>AAMAGGEGNMSASATETNARVFSLHLGATRVVYNPASSGETLTVINDQDYPMLVQSEVLSEDQKSPAPFVVTPPLFRLDGQQSSRLRIVRTGGEFPPDRESLQWICVKGIPPKEGDRWAEGKDGEKKADKVSLNVQLSVSSCIKLFVRPPAVKGRPDD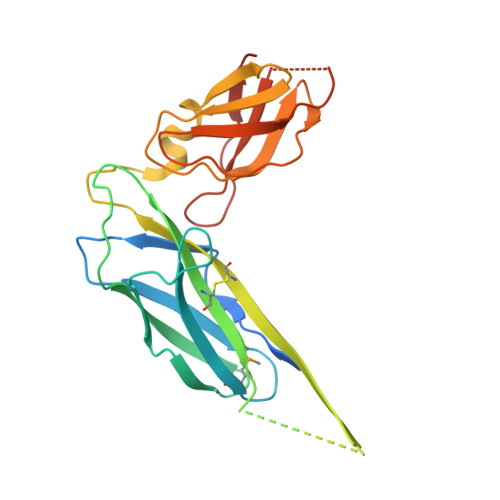VAGKVEWQRAGNRLKGVNPTPFYINLSTLTVGGKEVKEREYIAPFSSREYPLPAGASGKVQWKVITDYGGTSKQFEAELKG[8x]TRPV1-TRPV4 are non-selective cation channels which play important physiological roles in sensing noxious heat, maintaining cardiac structure and maintaining skin, hair and bone physiology. A distinctive feature of TRPV1 and TRPV2 is their permeability to large organic cations, such as the cationic dye YO-PRO-1 and the sodium channel blocker QX-314. The non-conducting structures of TRPV1 and TRPV2 possess two restrictions, one at the selectivity filter (SF) and second one at the intracellular mouth of the pore (termed the common gate). Our data shows that binding of RTx induces C2 symmetric conformations in TRPV2, but the extent of C2 symmetry depends on the environment in which the channel is reconstituted.

Classification of the TRPV2RTx-APOL sample revealed the presence of four classes: one low-resolution (~7 Å) class, which was excluded from further analysis, and three higher resolution classes which are representative of three different conformations. These include one C4 symmetric and two distinct C2 symmetric classes refined to 2.9 Å, 3.3 Å and 4.2 Å, respectively. Unexpectedly, the transmembrane domains (TM) of the three structures obtained from amphipol-reconstituted TRPV2, TRPV2RTx-APOL 1-3, show similarity to our previously solved cryo-EM structure of TRPV2 in its apo form (TRPV2APO) and adopt non-conducting conformations. While fully bound to RTx, the TM domains of TRPV2RTx-APOL 1 and TRPV2RTx-APOL 2 structures largely retain C4 symmetry. However, the TMs of TRPV2RTx-APOL 3 exhibit a slight departure from C4 symmetry in the pore. The effects of RTx on the TRPV2RTx-APOL are particularly obvious in the ankyrin repeat domains (ARD) of the two-fold symmetric TRPV2RTx-APOL 2 and TRPV2RTx-APOL 3 which display pronounced broken symmetry and a range of rotational states (Figure 3—figure supplements 1–3). Instead, RTx only effects changes in its immediate binding site above the S4-S5 linker and in the parts of the channel not bound by amphipol, strongly suggesting that the polymer constricts the TM and prevents conformational changes at the S4-S5 linker and the ARD from propagating to the TM domain. The fact that the TRPV2/RTx complex is stabilized in multiple distinct closed states with different arrangements of the ARD assembly (Figure 3—figure supplements 1–3) suggests that the conformational changes in the ARD might represent low-energy, pre-open states that can be achieved without substantial changes in the TM domains. Nevertheless, the RTx-induced conformational changes in the S4-S5 linker are not efficiently propagated to the TM in the TRPV2RTx-APOL structures, and they fail to open either of the two restrictions in the pore. As observed in our previous study, RTx assumes different binding poses in subunits of the C2-symmetric structures, both in the amphipol and the nanodisc samples which may lead to the distinct conformations observed in these channels.

>MTSPSSPPAFRLETSDGGQDGAEVDKAQLGYGAGPPPMESRFQDEDRNFPPQIKVNLNYRKGAGASQPDLNRFDRDRLFNVVARGNPEDLAGLLEYLRRTSKYLTDSEYTEGSTGKTCLMKAVLNLQDGVNACIQPLLEIDRDSGNPQPLVNAQCTDEYYRGHSALHIAIEKRSLQCVKLLVENGANVHAKACGHFFQKNQDTCFYFGELPLSLAACTKQWDVVNYLLENPHQPASLQAQDSLGNTVLHALVMIADDSAENSALVVRMYDGLLQAGARLCPNVQLEGIPNLEGLTPLKLAAKEGKIEIFKHILQREFSAPCQSLSRKFTEWCYGPVRVSLYDLASVDSWEENSVLEIIAFHSRSPHRHRMVVLEPLNKLLQAKWDRLIPRFCFNFLCYLVYMLIFTAVAYHQPALEKQGFPPLKATAGNSMLLLGHILILLGGVYLLLGQLWYFWRRRLFIWISFMDSYSEILFLLQALLTVLSQVLCFLAIEWYLPLLVSSLAMGWTNLLYYTRGFQHTGIYSVMIEKVILRDLLRFLLVYLVFLFGFAVALVSLSREAQNSRTPAGPNATEVGQPGAGQEDEAPPYRSILDASLELFKFTIGMGELAFQEQLRFRGVVLLLLLAYVLLTYVLLLNMLIALMSETVNSVATDSWSIWKLQKAISVLEMENGYWWCRRKKQRAGVMLTVGTRPDGSPDERWCFRVGEMNWATWEQTLPRTLCEEPSGAAAPGVMKNPTPASQRGEDSASEEDHLPLQLLQSRSNLEVLFQGPHHHHHHDYKDDDDK[4x]>ALFGYARVSTSQQSLDIQVRALKDAGVKANRIFTDKASGSSSDRKGLDLLRMKVKEGDVILVKKLDHLGRDTADMIQLIKEFDAQGVSIRFIDDGISTDSYIGKMVVTILSAVAQAERQRILERTNEGRQEAMHHHH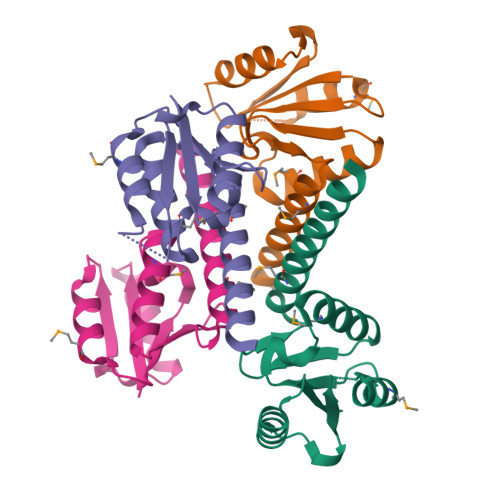HH[4x]Mtb GlgE is a genetically validated anti-TB target as the absence of Mtb GlgE leads to cytosolic accumulation of toxic levels of M1P by a self-amplifying feedback response leading to cell death. Previously, we have shown that hydroxypyrrolidines modified with an α-configured − 2 site sugar can inhibit Mtb GlgE (Ki = 237 ± 27 µM) as well Sco GlgE1-V279S (Ki = 102 ± 7 µM), a closely related homolog from Streptomyces coelicolor (Sco) GlgE1 that has been mutated to be 100% identical to the M1P binding site of Mtb GlgE, and affords much higher quality X-ray diffraction data.

Enzyme activity of Sco GlgE1-V279S decreased by 32% at 100 µM concentration of 8, but 7 failed to exhibit any inhibition of Sco GlgE1-V279S. Although 7 failed to inhibit the activity of Sco GlgE1-V279S in the reaction conditions described here, we thought to examine any interactions formed between 7 and the enzyme that may inform future drug design by identifying interactions between enzyme and ligand that destabilize the Sco GlgE1-V279S/7 complex. In addition to the strong density observed for both 7 and 8 in the respective structures, the GlgE1-V279S/7 complex also exhibits a well-ordered spherical density located 3.2 Å from the exocyclic amine moiety of 7 that we have modeled as a chloride ion. The location of the chloride ion overlaps significantly with that of negatively charged phosphate and phosphonate moieties in previous GlgE1-V279S crystal structures. In the Sco GlgE1-V279S/7 complex, the interactions are similar to those observed in the substrate-bound (M1P and maltose) and substrate-mimic (MCP) complexes because the saturated carbocycle in 7 maintains the expected chair conformation. Specifically, the C(2)–OH and C(3)–OH functional groups form a bidentate hydrogen-bonded interaction with Asp 480, which is a unique feature to the GH13 family of proteins and has been observed previously in GlgE. An unexpected difference between the Sco GlgE1-V279S/7 complex structure and other complexes of disaccharide-like compounds is the rotation of the Asp 394 side chain away from the substrate analog. Due to this bond rotation, Asp 394 in Sco GlgE1-V279S shifts away from the substrate binding site and does not form any direct interaction with 7. While this structural change in Asp 394 is exhibited unambiguously by the 2FO − FC composite omit map density contoured at 1.5σ, the reason for this movement of Asp 394 appears to derive from steric hindrance with atom C(1) of 7 apparently due to the attraction between the C(1) ammonium moiety and the Glu 423 side chain. However, the very short distance between those atoms can be rationalized if either of the two side chains becomes protonated and the O(D1) atoms in those residues are using that hydrogen in a low barrier hydrogen bond.

>[2x]MPATHHSSATSAERPTVVGRIPVLDVRPVVQRGRRPAKAVTGESFEVSATVFREGHDAVGANVVLRDPRGRPGPWTPMRELAPGTDRWGATVTAGETGTWSYTVEAWGDPVTTWRHHARIKIPAGLDTDLVLEEGARLYERAAADVPGREDRRELLAAVDALRDESRPAASRLAAALTPQVDAVLARHPLRDLVTSSDPLPLLVERERALYGAWYEFFPRSEGTPHTPHGTFRTAARRLPAIAAMGFDVVYLPPIHPIGTTHRKGRNNTLSATGDDVGSPWAIGSPEGGHDSIHPALGTLDDFDHFVTEAGKLGLEIALDFALQCSPDHPWVHKHPEWFHHRPDGTIAHAENPPKKYQDIYPIAFDADPDGLATETVRILRHWMDHGVRIFRVDNPHTKPVAFWERVIADINGTDPDVIFLAEAFTRPAMMATLAQIGFQQSYTYFTWRNTKQELTEYLTELSGEAASYMRPNFFANTPDILHAYLQHGGRPAFEVRAVLAATLSPTWGIYSGYELCENTPLREGSEEYLDSEKYQLKPRDWTRAAREGTTIAPLVTRLNTIRRENPALRQLRDLHFHPTDKEEVIAYSKRQGSNTVLVVVNLDPRHTQEATVSLDMPQLGLDWHESVPVRDELTGETYHWGRANYVRLEPGRTPAHVCTVLRPSHPQIGGSHTTALHHHHHH>[2x]MSNKCDVVVVGGGISGMAAAKLLHDSGLNVVVLEARDRVGGRTYTLRN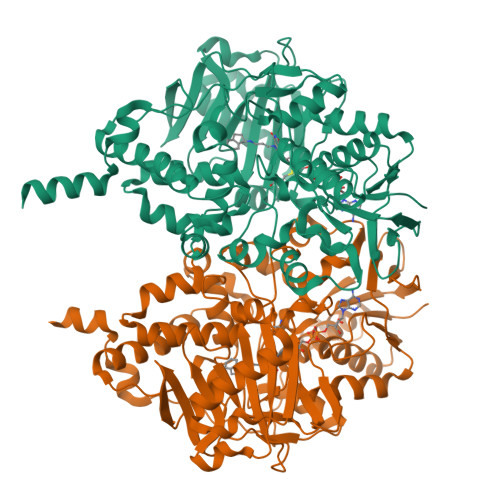QKVKYVDLGGSYVGPTQNRILRLAKELGLETYKVNEVERLIHHVKGKSYPFRGPFPPVWNPITYLDHNNFWRTMDDMGREIPSDAPWKAPLAEEWDNMTMKELLDKLCWTESAKQLATLFVNLCVTAETHEVSALWFLWYVKQCGGTTRIFSTTNGGQERKFVGGSGQVSERIMDLLGDRVKLERPVIYIDQTRENVLVETLNHEMYEAKYVISAIPPTLGMKIHFNPPLPMMRNQMITRVPLGSVIKCIVYYKEPFWRKKDYCGTMIIDGEEAPVAYTLDDTKPEGNYAAIMGFILAHKARKLARLTKEERLKKLCELYAKVLGSLEALEPVHYEEKNWCEEQYSGGCYTTYFPPGILTQYGRVLRQPVDRIYFAGTETATHWSGYMEGAVEAGERAAREILHAMGKIPEDEIWQSEPESVDVPAQPITTTFLERHLPSVPGLLRLIGLTTIFSATALGFLAHKRGLLVRV(1R)-2-{[(S)-(2-aminoethoxy)(hydroxy)phosphoryl]oxy}-1-[(pentadecanoyloxy)methyl]ethyl (12E)-hexadeca-9,12-dienoate | C36 H68 N O8 P | 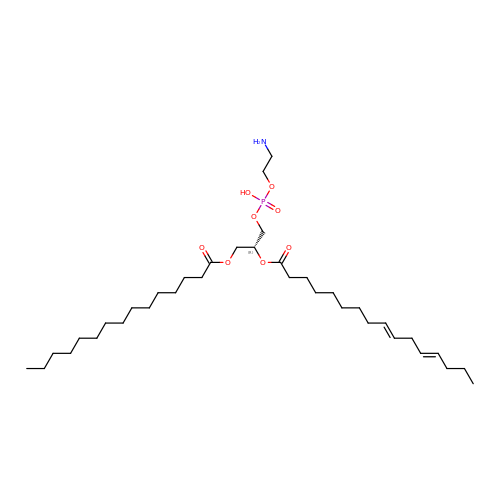NMIBJXZODRRZEA-NTSPIXPOSA-N> SNAMEPEMHFDLSSEPWLPVRFRDGRRSEVSLRDIFVLAHTIVGFDVDFPTLEPALLRLVLALAYRILRGPKDDAEWGRLWEADRFSEDAIDDYFARWRHRFDLFSKEFPFFQVADLEPAGKGGVKTANSLVAYAPSGNNVPVFTPITDRTELALSPAEAARWLVERHAFGSASDKTGAKGNPKVKGGKDTPAIGYLAWIGFVAPVGQTLRETLLLNLVPWQYRNLIRGGEDDVPAWERDPLGPTRVMRAPDGVCDLFTWQGRRIRLFPERRGDAIVVPRVLICAGDEVDRRAARDVDPHVGWRMESRRGAEVSYVPLRARPGQQVWRGLSSVLALGAEEQRAGVLSFVEGLQSRGIALVSLLVTSAKFGNMSTTLDDLAYDRLDTPLAVLNQEDPAAATVAIDAVTFAAHAAQALGYVAEARYLSYDLSFHEESKRHRVPEGKAALAKAARSALAEEIYGRLDAPYRHFLTGLANIDDLERPRAEWAALVEAVARDLASRELAQ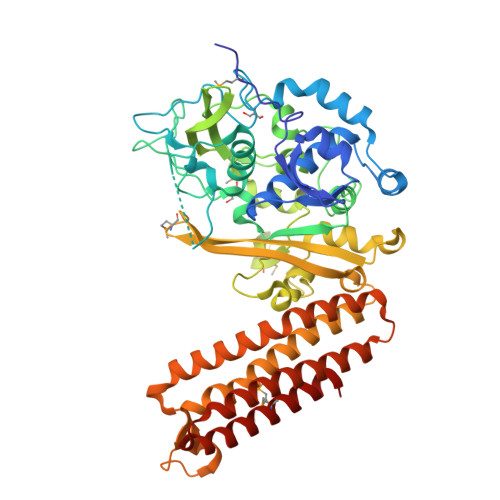LAPAQAFAGVAGEDRFRRMLARARNEFSPSDSPEKGAA>[4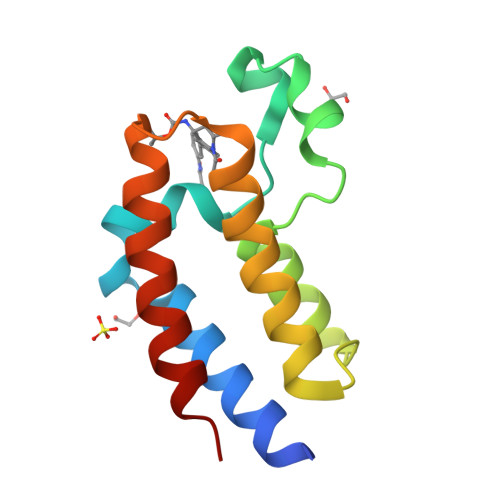x]SMGKLSEQLKHCNGILKELLSKKHAAYAWPFYKPVDASALGLHDYHDIIKHPMDLSTVKRKMENRDYRDAQEFAADVRLMFSNCYKYNPPDHDVVAMARKLQDVFEFRYAKMPD>[8x]MEVKIGITDSPRE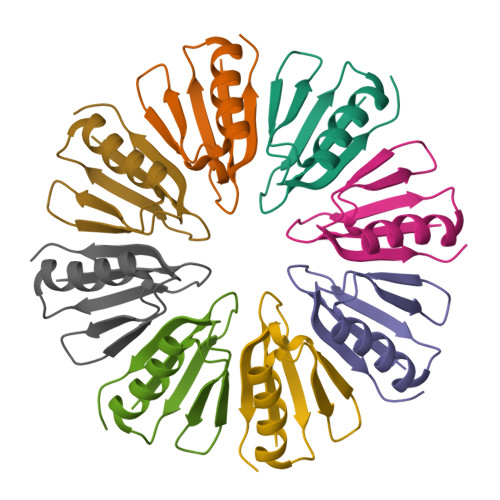LVFSSAQTPSEVEELVSNALRDDSGLLTLTDERGRRFLIHTARIAYVEIGVADARRVGFGVGVDAAAGSAGKVATSG[3-(4-amino-6-methyl-1H-imidazo[4,5-c]pyridin-1-yl)-3-methylazetidin-1-yl][1-({1-[(1R)-cyclohept-2-en-1-yl]piperidin-4-yl}methyl)-1H-pyrrol-3-yl]methanone | C29 H39 N7 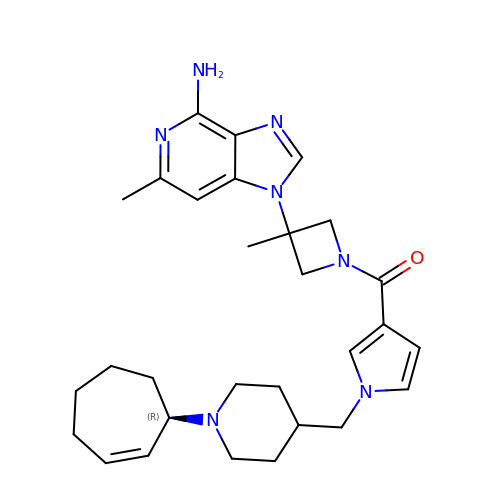O | AVKAVKZKOFSSMY-DEOSSOPVSA-N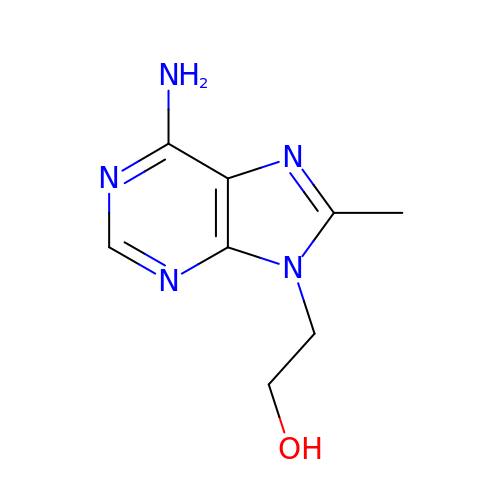2-(6-azanyl-8-methyl-purin-9-yl)ethanol | C8 H11 N5 O | JSYNJZZGNMUJED-UHFFFAOYSA-N>[2x]SNAMRQRTIVCPLIENEGHYLLCKMAADRGVFPGQWALSGGGVEPGERIEEALRREIREELGEKLILTHIAPWCFRDDTRVKTYPDGHQET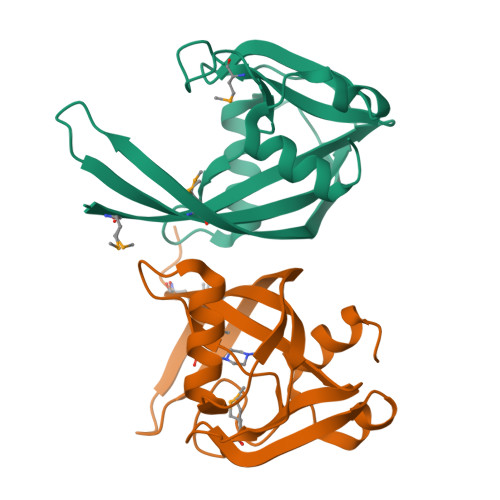IYMIYLIFNCVSANRDVTINEEFDDYAWVKAEDLKNYDLNAATRVTLSLKGLL>ADPGMDEITITTQPKSGYVIRNKPLRLQCRANHATKIRYKCSSKWIDDSRIEKLIGTDSTSGVGYIDASVDISRIDVDTSGHVDAFQCQCYASGDDDQDVVASDVATVHLAYMRKHFLKSPVAQRVQEGTTLQLPCQA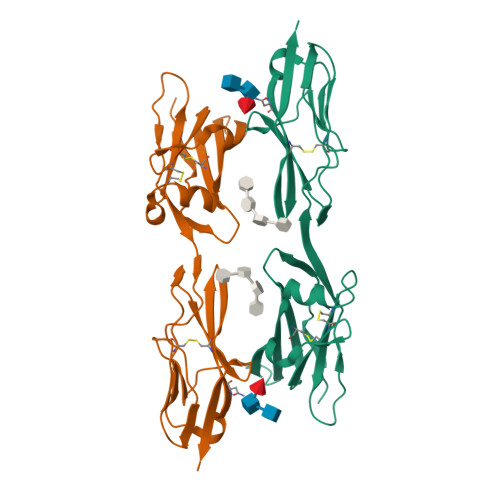PESDPKAELTWYKDGVVVQPDANVIRASDGSLIMSAARLSDSGNYTCEATNVANSRKTDPVEVQIYHHHHHH[2x]>MARRLPKPTLQGRLEADFPDSPLLPKFQELNQNNLPNDVFREAQRSYLVFLTSQFCYEEYVQRTFGVPRRQRAIDKRQRASVAGAGAHAHLGGSSATPVQQAQAAASAGTGALASSAPSTAVAQSATPSVSSSISSLRAATSGATAAASAAAAVDTGSGGGGQPHDTAPRGARKKQ[4x];>MKVQGSVDRRRLQRRIAGLLPPPARRLNISRGSEFTRDVRGLVEEHAQASSLSAAAVWRAGLLAPGEVAVAGGGSGGGSFSWSGWRPPVFGDFLIHASSFNNAEATGTPLFQFKQSDPFSGVDAVFTPLSLFILMNHGRGVAARVEAGGGLTRMANLLYDSPATLADLVPDFGRLVADRRFHNFITPVGPLVENIKSTYLNKITTVVHGPVVSKAIPRSTVKVTVPQEAFVDLDAWLSGGAGGGGGVCFVGGLGLQPCPADARLYVALTYEEAGPRFTFFQSSRGHCQIMNILRIYYSPSIMHRYAVVQPLHIEELTFGAVACLGTFSATDGWRRSAFNYRGSSLPVVEIDSFYSNVSDWEVIL[2x];>[4x]MDLKVVVSLSSRLYTDEIAKMQQRIGCILPLASTHGTQNVQGLGLGQVYSLETVPDYVSMYNYLSDCTLAVLDEVSVDSLILTKIVPGQTYAIKNKYQPFFQWHGTGSLSVMPPVFGREHATVKLESNDVDIVFPMVLPTPIAEEVLQKILLFNVYSRVVMQAPGNADMLDVHMHLGSVSYLGHHYELALPEVPGPLGLALLDNLSLYFCIMVTLLPRASMRLVRGLIRHEHHDLLNLFQEMVPDEIARIDLDDLSVADDLSRMRVMMTYLQSLASLFNLGPRLATAAYSQETLTATCWLR;>[2x]MSNGDWGQSQRTRGTGPVRGIRTMDVNAPGGGSGGSALRILGTASCNQAHCKFGRFAGIQCVSNCVLYLVKSFLAGRPLTSRPELDEVLDEGARLDALMRQSGILKGHEMAQLTDVPSSVVLRGGGRVHIYRSAEIFGLVLFPAQIANSAVVQSLAEVLHGSYNGVAQFILYICDIYAGAIIIETDGSFYLFDPHCQKDAAPGTPAHVRVSTYAHDILQYVGAPGAQYTCVHLYFLPEAFETEDPRIFMLEHYGVYDFYEANGSGFDLVGPELVSSDGEAAGTPGADSSPPVMLPFERRIIPYNLRPLPSRSFTSDSFPAARYSPAKTNSPPSSPASAAPASAAPASAAPASAAPASAAPASAAPASAAPASAAPASSPPLFIPIPGLGHTPGVPAPSTPPRASSGAAPQTPKRKKGLGKDSPHKKPTSGRRLPLSSTTDTEDDQLPRTHVPPHRPPSAARLPPPVIPIPHQSPPASPTPHPAPVSTIAPSVTPSPRLPLQIPIPLPQAAPSNPKIPLTTPSPSPTAAAAPTTTTLSPPPTQQQPPQSAAPAPSPLLPQQQPTPSAAPAPSPLLPQQQPPPSAARAPSPLPPQQQPLPSATPAPPPAQQLPPSATTLEPEKNHPPAADRAGTEISPSPPFGQQPSFGDDASGGSGLVRYLSDLEEPFLSMSDSEEAESDLASDIPTTEDEDMFEDEVFSNSLESGSSAPTSPITLDTARSQYYQTTFDIETPEMDFVPLESNIARIAGHTYQEQAIVYDPASNREVPEADALSMIDYLLVTVVLEQGLIRSRDRSSVLNLLEFLKDWSGHLQVPTLDLEQLLTSELNIQNLANMLSENKGRAGEFHKHLAAKLEACLPSLATKDAVRVDAGAKMLAEIPQLAESDDGKFDLEAARRRLTDLLSGGDQEAGEGGGEPEDNSIYRGPHVDVPLVLDDESWKRLLSLAEAARTAVARQQAGVDEEDVRFLALLTAIEYGAPPAASVPPFVHNVAVRSKNAALHVRRCTADIRDKVASAASDYLSYLEDPSLPTVMDFDDLLTHLRHTCQIIASLPLLNIRYTSIEWDYRELLYLGTALSDMSGIPWPLERVEEDDPSIAPLPEFETVAKKQKELETTRENEKRLRTILDDIEAMLGLAGVASAPGAPISPASPSATPANHDNPEATPPLADTAALTIPVIEKYIANAGSIVGAAKNPTYIRLRDTIQQIVRSKKYLMNILKSITFYTIDNYIASFEESIDHLYRDLPVLDPEVQDGIDRILDPMVSEALHTFEMGNRLTLEPARLVALQNFATHSTLKETAAAVNLLPGLLAVYDATITGQAPEDALRLLSGLQNQLSQTLIPGKLKKRFLSYLQKLKNNNNDQLRQKEVQAWRLEAEGFKPATEEQLEAFLDTAPNKELKRQYEKKLRQLMETGRKEKEKLREQEDKERQERRAREANEAWARIRKALGARPEPAPTSPDDWNTLLASLLPDNTDSAAAAAAAVARNTDILDSLTQILAAMLLGITRVRRERLRSLLVDDGGAAERMEAAEPGWFTDIETGPLARLDAWPATPAATAKEGGGGRGAEEAAGALFRARTAADAIRSALAQTRQALQSPDMKSAVVNTDLEAPYAEYERGLAGLLEKRRAAEAALTAIVSEYVDRTLPEATNDPGQANLPPPPTIPQATAPPRLASDSALWPKKPQLLTRRERDDLLQATGDFFSELLTEAEAAEVRALEEQVRESQTLMAKAHEMAASTRRGFHTALEAVLSRSRDEAPDDELRSLLPSPPKAPVQAPLEAALARAAAGNGSWPYRKSLAAAKWIRGICEAVRGLSEGALALAGGAGAWLNLAAAADGEIHELTRLLEVEGMAQNSMDGMEELRLALATLDPKRVAGGKETVADWKRRLSRLEAIIQEAQEESQLQGTLQDLVTQARGHTDPRQLKIVVEAARGLALGASAGSQYALLKDKLLRYASAKQSFLAFYETAQPTVFVKHPLTNNLPLLITISAPPTGWGNGAPTRRAQFLAAAGPAKYAGTLWLETESPCDPLNPAYVSADTQEPLNYIPVYHNFLEYVMPTVLENPEAFSLTPAGRPQAIGPPQDDQERRRRTLASVASARLSAAAADSYWDTWPDVESNAGELLREYVSAPKALMEDLADNPIVAMTLLAHASLIASRNHPPYPAPATDREVILLEQREMMALLVGTHPAYAAAFLGAPSFYAGLGLVSALARDGGLGDLLSDSVLTYRLVRSPASGRGGMPSTTRGSNDGEDARRLTRHRIAGPPTGFIFFQDAWEEMDTRAALWPHPEFLGLVHNQSTARARACMLLLARRCFAPEALQQLWHSLRPLEGPVAFQDYLRDFVKQAYTRGEELPRAEGLEVPRETPSSYGTVTGRALRNLMPYGTPITGPKRGSGDTIPVSVFEAAVAAAFLGRPLTLFVSSQYLFNLKTLGQVRVVAPLLYCDGHSEPFRSLVETISLNFLQDLDGYSESFEPEMSIFARQAVWLRELLTEARAAKPKEARPPTVAILANRKNIIWKCFTYRHNLPDVQFYFNAAGASRWPTDVLNPSFYEHEDPPLPVGYQLPPNPRNVQELFSGFPPRVGHGLVSGDGFQSADNTPASSDRLQQLGGGETDQGEKGSTTAESEASGPPSPQSPLLEKVAPGRPRDWLSPTSSPRDVTVTPGLAAPITLPGPRLMARPYFGAETRASESPDRSPGSSPRPWPKDSLELLPQPAPQQPPSSPWASEQGPIVYTLSPHSTPSTASGSQKKHTIQIPGLVPSQKPSYPPSAPYKPGQSTGGIAPTPSAASLTTFGLQPQDTQASSQDPPYGHSIMQREKKQQGGREEAAEIRPSATRLPTAVGLRPRAPVVAAGAAASATPAFDPGEAPSGFPIPQAPALGSGLAAPAHTPVGALAPRPQKTQAQRPQDAAALPTPTIKAVGARPVPKATGALAAGARPRGQPTAAPPSAASPPRVSLPVRSRQQQSPAIPLPPMHSGSEPGARPEVRLSQYRHAGPQTYTVRKEAPPSAASQLPKMPKCKDSMYYPPSGSARYPAPFQALSFSQSVASPAPSSDQTTLLWNTPSVVTQFLSIEDIIREVVTGGSTSGDLVVPSGSPSSLSTAAPEQDLRYSLTLSQASRVLSRFVSQLRRKLERSTHRLIADLERLKFLYL;> MDVHIDNQVLSGLGTPLLVHLFVPDTVMAELCPNRVPNCEGAWCQTLFSDRTGLTRVCRVFAARGMLPGRPSHRGTFTSVPVYCDEGLPELYNPFHVAALRFYDEGGLVGELQIYYLSLFEGAKRALTDGHLIREASGVQESAAAMQPIPIDPGPPGGAGIEHMPVAAAQVEHPKTYDLKQILLEITQEENRGEQRLGHAGSPALCLGLRLRAGAETKAAAETSVSKHHPALENPSNIRGSAGGEGGGGRAGTGGTVGVGSGALSRVPVSFSKTRRAIRESRALVRGIAHIFSPHALYVVTYPELSAQGRLHRMTAVTHASPATDLAEVSILGAPEREFRFLISVALRISASFREKLAMQAWTAQQEIPVVIPTSYSRIYKNSDLIREAFFTVQTRVSWESCWVKATISNAPKTPDACLWI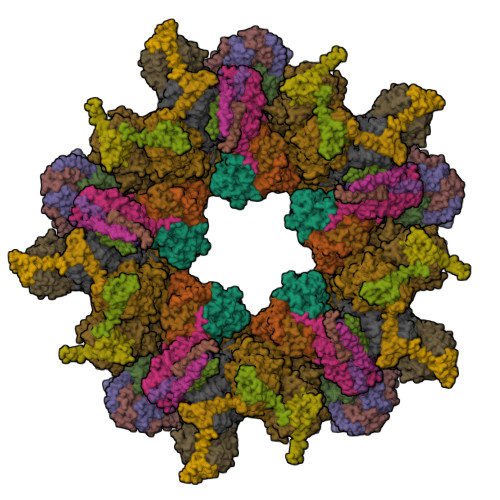DSHPLYEEGASAWGKVIDSRPPGGLVGAASQLVALGTDGHCVHLATTSDGQAFLVLPGGFVIKGQLALTPEERGYILARHGIRREQ;>MALSGHVLIDPARLPRDTGPELMWAPSLRNSLRVSPEALELAEREAERARSERWDRCAQVLKNRLLRVELDGIMRDHLARAEEIRQDLDAVVAFSDGLESMQVRSPSTGGRSAPAPPSPSPAQPFTRLTGNAQYAVSISPTDPPLMVAGSLAQTLLGNLYGNINQWVPSFGPWYRTMSANAMQRRVFPKQLRGNLNFTNSVSLKLMTEVVAVLEGTTQDFFSDVRHLPDLQAALILSVAYLLLQGGSSHQQRPLPASREELLELGPESLEKIIADLKAKSPGGNFMILTSGNKEARQSIAPLNRQAAYPPGTFADNKIYNLFVGAGLLPTTAALNVPGAAGRDRDLVYRIANQIFGEDVPPFSSHQWNLRVGLAALEALMLVYTLCETANLAEAATRRLHLSSLLPQAMQRRKPAMASAGMPGAYPVQTLFRHGELFRFIWAHYVRPTVAADPQASISSLFPGLVLLALELKLMDGQAPSHYAINLTGQKFDTLFEIINQKLLFHDPAAMLAARTQLRLAFEDGVGVALGRPSPMLAAREILERQFSASDDYDRLYFLTLGYLASPVAPS[2x];>MASNEGVENRPFPYLTVDADLLSNLRQSAAEGLFHSFDLLVGKDAREAGIKFEVLLGVYTNAIQYVRFLETALAVSCVNTEFKDLSRMIDGKIQFRISVPTIAHGDGRRPSKQRTFIVVKNCHKHHISTEMELSMLDLEILHSIPETPVEYAEYVGAVKTVASALQFGVDALERGLINTVLSVKLRHAPPMFILQTLADPTFTERGFSKTVKSDLIAMFKRHLLEHSFFLDRAENMGSGFSQYVRSRLSEMVAAVSGESVLKGVSTYTTAKGGEPVGGVFIVTDNVLRQLLTFLGEEADNQIMGPSSYASFVVRGENLVTAVSYGRVMRTFEHFMARIVDSPEKAGSTKSDLPAVAAGVEDQPRVPISAAVIKLGNHAVAVESLQKMYNDTQSPYPLNRRMQYSYYFPVGLFMPNPKYTTSAAIKMLDNPTQQLPVEAWIVNKNNLLLAFNLQNALKVLCHPRLHTPAHTLNSLNAAPAPRDRRETYSLQHRRPNHMNVLVIVDEFYDNKYAAPVTDIALKCGLPTEDFLHPSNYDLLRLELHPLYDIYIGRDAGERARHRAVHRLMVGNLPTPLAPAAFQEARGQQFETATSLAHVVDQAVIETVQDTAYDTAYPAFFYVVEAMIHGFEEKFVMNVPLVSLCINTYWERSGRLAFVNSFSMIKFICRHLGNNAISKEAYSMYRKIYGELIALEQALMRLAGSDVVGDESVGQYVCALLDPNLLPPVAYTDIFTHLLTVSDRAPQIIIGNEVYADTLAAPQFIERVGNMDEMAAQFVALYGYRVNGDHDHDFRLHLGPYVDEGHADVLEKIFYYVFLPTCTNAHMCGLGVDFQHVAQTLAYNGPAFSHHFTRDEDILDNLENGTLRDLLEISDLRPTVGMIRDLSASFMTCPTFTRAVRVSVDNDVTQQLAPNPADKRTEQTVLVNGLVAFAFSERTRAVTQCLFHAIPFHMFYGDPRVAATMHQDVATFVMRNPQQRAVEAFNRPEQLFAEYREWHRSPMGKYAAECLPSLVSISGMTAMHIKMSPMAYIAQAKLKIHPGVAMTVVRTDEILSENILFSSRASTSMFIGTPNVSRREARVDAVTFEVHHEMASIDTGLSYSSTMTPARVAAITTDMGIHTQDFFSVFPAEAFGNQQVNDYIKAKVGAQRNGTLLRDPRTYLAGMTNVNGAPGLCHGQQATCEIIVTPVTADVAYFQKSNSPRGRAACVVSCENYNQEVAEGLIYDHSRPDAAYEYRSTVNPWASQLGSLGDIMYNSSYRQTAVPGLYSPCRAFFNKEELLRNNRGLYNMVNEYSQRLGGHPATSNTEVQFVVIAGTDVFLEQPCSFLQEAFPALSASSRALIDEFMSVKQTHAPIHYGHYIIEEVAPVRRILKFGNKVVF[4x]>[3x]NRRNKARKVVSRSTALVPMAPASQRTGPAPRKPRKRNQALVRNPRLTDAGLAFLKCAFAAPDFSVDPGKGIPDNFHGRTLAIKDCNTTSVVFTPNTDTYIVVAPVPGFAYFRAEVAVGAQPTTFVGVPYPTYATNFGAGSQNGLPAVNNYSKFRYASMACGLYPTSNMMQFSGSVQVWRVDLNLSEAVNPAVTAITPAPGVFANFVDKRINGLRGIRPLAPRDNYSGNFIDGAYTFAFDKSTDFE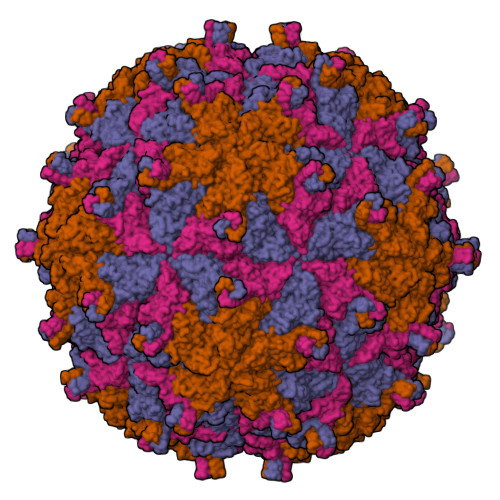WCDFVRSLEFSESNVLGAATAMKLLAPGGGTDTTLTGLGNVNTLVYKISTPTGAVNTAILRTWNCIELQPYTDSALFQFSGVSPPFDPLALECYHNLKMRFPVAVSSREN;>[3x]SKFWEGVLRVLNQISGTLSVIPGPVGTISAGVHQLTGMYM> ALLDETPLPPGSRLDVRAYTTVLHALSRAGRYERALELFAELRRQGVAPTVVTYNTLIDGLCKAGKLDEALKLFEEMVEKGIKPDVVTYNTLIDGLCKAGKLDEALKLFEEMVEKGIKPDVVTYNTLIDGLCKAGKLDEALKLFEEMVEKGIKPDVVTYNTLIDGLCKAGKLDEALKLFEEMVEKGIKPDVVTYTTLIDGLCKAGKLDEALKLFEEMVEKGIKPDVVTYTTLIDGLCKAGKLDEALKLFEEMVEKGIKPDVVTYNTLIDGLCKAGKLDEALKLFEEMVEKGIKPDVVTYNTLIDGLCKAGKLDEALKLFEEMVEKGIKPDVVTYNTLIDGLCKAGKLDEALKLFEEMVEKGIKPDVVTYNTLIDGLCKAGKLDEALKLFEEMVEKGIKPDELTYRRVVESYCRAKRFEEARGFLSEVSETDLDFDKKALEAYIEDAQFGRLEHHHHHHHH

Containing a tandem array of 2–30 repeats, pentatricopeptide repeat (PPR) proteins constitute one of the largest protein families in land plants. Each PPR repeat aligns to a single nucleotide of the RNA target in modular patterns, making these proteins suitable for the development of exciting new biotechnologies. Within each repeat, the combinations of two amino acids, known as the PPR code at two key positions (the 5th and the 35th) confer RNA specificity. A typical RNA-bound dPPR protein adopts a right-handed superhelical spiral structure, with its target ssRNA molecule sitting in the interior cavity and interacting with corresponding PPR repeats in a modular fashion.

To verify the RNA selectivity, the dPPR proteins dPPR-U8N2 (in which N indicates any nucleotide) comprising 10 dPPR repeats with different 5th and 6th repeats with different PPR codes were constructed and purified to homogeneity. After numerous unsuccessful trials, we finally succeeded in crystallizing each dPPR-U8N2 in complex with its respective target ssRNA (5′-UUUUNNUUUU-3′), in space group P212121. When dPPR-U8C2 was superimposed on dPPR-U10, dPPR-U8A2 and dPPR-U8G2, the root mean square deviations were 0.73, 0.99 and 1.00 Å over 348, 367 and 374 Cα atoms, respectively. As observed in all four complex structures, four types of dPPR repeats recognize their corresponding targets by forming hydrogen bonds with the Watson–Crick faces of the nucleotides, which explains why PPR proteins bind ssRNAs instead of double stranded ones. Serine or threonine at this position results in a preference for purines, whereas the presence of asparagine is correlated with a preference for pyrimidines. The amide group of the Asn5 side chain donates a hydrogen bond to the O2 atom of the corresponding pyrimidine, whereas the N3 atom of purine accepts a hydrogen bond from the hydroxyl group of the corresponding amino acid. For purine, Asn35 or Asp35 form one or two hydrogen bonds with adenine and guanine, respectively. The N1 atom of adenine is a hydrogen bond acceptor, whereas both the N1 and N2 atoms of guanine are hydrogen bond donors. These structures demonstrate how the amino acids asparagine and aspartate at the 35th position contribute to purine base selectivity.> SASSSDSDLSDFASSVLAEHNKKRALHKDTPALSWSDTLASYAQDYADNYDCSGTLTHSGGPYGENLALGYDGPAAVDAWYNEISNYDFSNPGFSSNTGHFTQVVWKSTTQVGCGIKTCGGAWGDYVICSYDPAGNYEGEYADNVEPLA

Two crystal structures of the CAP domain of pathogen-related yeast protein from Saccharomyces cerevisiae, Pry1CAP, are presented. Our previous studies revealed that Saccharomyces cerevisiae CAP proteins are required for the export of sterols in vivo and they bind cholesterol in vitro. The sterol binding and export properties of these proteins are localized to the CAP domain, which is sufficient to rescue sterol export properties of cells lacking endogenous Pry proteins. The overall monomer surface area for Pry1CAP is 7125 Å2 and its topology is an alpha-beta-alpha sandwich made up of 6 helices, 2 disulfide bonds, 12 beta turns and 1 beta bulge.

Electron density for four 1,4-dioxane molecules were observed in the initial molecular replacement 2Fo − Fc maps when dioxane was present in the crystallization solution; this density is absent in the Mg2+ structure, which does not have 1,4-dioxane in the crystallization solution. Density corresponding to one 1,4-dioxane molecule was observed in the 194 Å3 volume cavity created by the CBM, confirming for the first time the ability of the cholesterol binding site of Pry1 to bind a ligand. In one structure a 1,4-dioxane molecule from the crystallization mixture occupies the CBM cavity confirming its ability to bind hydrophobic ligands. Since a 1,4-dioxane molecule binds to the CBM cavity, and the CBM is verified to be important for cholesterol binding, the effect of 1,4-dioxane on cholesterol binding was tested. 1,4-dioxane inhibits in vitro binding of [3H]-cholesterol to Pry1CAP in a dose dependent manner. However, the inhibition was only observed at relatively high concentrations of 1,4-dioxane, and is possibly due to the increased hydrophobicity of the 1,4-dioxane containing solvent compared to the aqueous buffer. Interestingly, 1,4-dioxane does not bind to other lipid binding sites notably the palmitate binding site of Tablysin-1519 or phosphatidylinositol binding sites of GAPR-12324. The presence of dioxane in the crystallization solution was incompatible with the formation of complexes of Pry1CAP with cholesterol or palmitate and all co-crystallization and soaking experiments yielded crystals with dioxane only. Mg2+ dependent sterol binding by Pry1CAP requires the interaction of both binding sites, likely occuring via dimerization, because Pry1CAP forms dimers in solution, and both crystal structures have a crystallographic dimer in which the CBM and CAP tetrad are connected within a large 7063 Å3 volume cleft.L-METHIONYL ADENYLATE | C15 H27 N6 O7 P S | 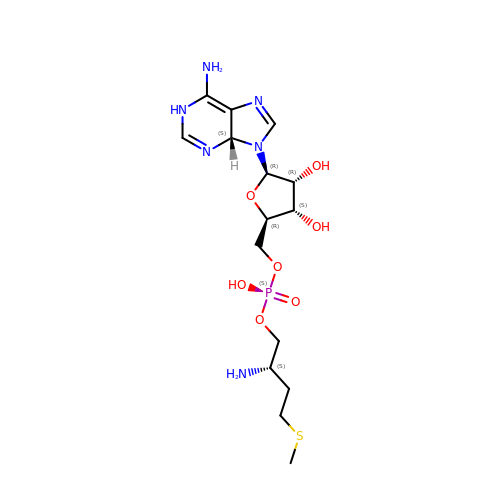GJUQRKWTINGHCW-LLTXIYJVSA-N In E. coli, the ssuABC and tauABC gene products encode for an ABC transporter for the uptake of alkanesulfonates and taurine, respectively; TauA is the SBP that recognizes and binds taurine, TauBC is the ABC transporter that mediates the transport of taurine in an ATP-dependent manner. The SsuA and TauA proteins belong to the class II SBPs that are characterized by two globular domains, linked by a flexible linker, that form a cleft where the substrate binds. TauA is composed of two α/β-domains (domain I (23–104 and 202–319) and domain II (105–201)) connected by two-loop hinge regions (103–106 and 200–202) with the substrate-binding site located at the interface of the two domains; both domains are composed of five β-strands flanked by 11 and 4 α-helices, respectively. Although, SBPs are usually described as highly specific for their substrate, we show that TauA is capable of binding different taurine analogues and alkanesulfonates, including phosphonate analogues, with different affinities.

We also investigated if larger compounds such as the N-(2-acetamido)-2-aminoethanesulfonic acid (ACES) analogue, that has an acetamido group after the ethylamine group of taurine, and 2-(N-morpholino)ethanesulfonate (MES), that contains a morpholino group, could bind to TauA; we measured an apparent affinity of 7.4 µM and 2.8 µM, respectively. In light of the binding data, we co-crystallized TauA with 2-AEP, ACES and MES and collected X-ray data at 1.62 Å, 1.5 Å and 1.55 Å resolution, respectively. Inspection of electron density maps revealed electron density for 2-AEP, ACES and MES. The ACES with its longer acetamido group displays similar interactions as the taurine complex but its amine group is making additional hydrogen bonds to Asp84, whereas Asp84 in the taurine complex is bound to a water molecule, and its acetamido group is stabilized by hydrogen bonds between the side chain of Asn55 and the main chain amine of Ser10. In the taurine complex, the site occupied by the acetamido group is hydrated. The crystal structures of TauA with 2-AEP and ACES appear to be in ‘disagreement’ with the ITC data since the structures show that these molecules have formed more hydrogen bonds relative to taurine, they display much weaker affinities. Our structures show that upon ligand binding some waters have to be displaced to accommodate the larger alkanesulfonates such as ACES and MES. We also propose that desolvation of the binding site, loss of water molecules, contributes to the lower affinity for ACES and MES over taurine, although they display more hydrogen bonds than taurine.

>[2x]MVNVTVAYQTSAEPAKVAQADNTFAKESGATVDWRKFDSGASIVRALASGDVQIGNLGSSPLAVAASQQVPIEVFLLASKLGNSEALVVKKTISKPEDLIGKRIAVPFISTTHYSLLAALKHWGIKPGQVEIVNLQPPAIIAAWQRGDIDGAYVWAPAVNALEKDGKVLTDSEQVGQWGAPTLDVWVVRKDFAEKHPEVVKAFAKSAIDAQQPYIANPDVWLKQPENISKLARLSGVPEGDVPGLVKGNTYLTPQQQTAELTGPVNKAIIDTAQFLKEQGKVPAVANDYSQYVTSRFV>HHHHHHAGFIEDSKASLTLRNFYINTDNRNGTASPSKQEEWGQGFILNYQSGFTQGTVGFGVDALGLLGVRLDGGGRAGKSGLDRQPGTVFPLESNGEPVHDFASLGLTAKAKVSNTEFRYGTLQPKLPVVTYNDGRLLPVTFEGGQVTSTDLKDFTLVAGQLEHSKGRNSTDNRSLSIAGANGSSASSRDSNKFYYAGGDYKVNKDLTLQYYYGNLDDFYKQHFLGLIHNWQIGPGVLKTDLRAFDSSSDGKNGSRSGRADGYVSSGYYGSGVTKGEVDNRAFSGLFTYTV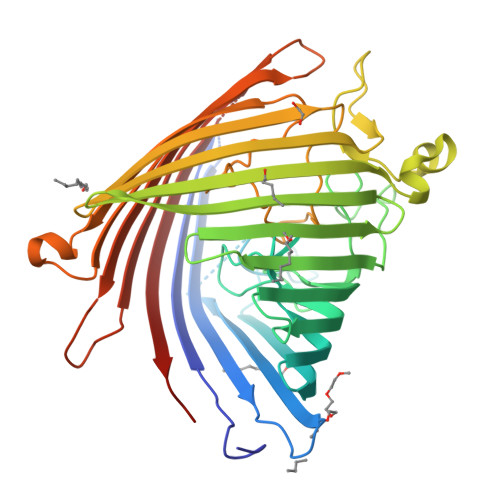SGHSIGAGYQILNGDSDFPFLNRGDGEGSTAYLITDVQIGKFQRAGERTWQVRYGYDFATVGVPGLTFNTIYLSGDKIKTARGDQSEWERDISLAYVIPDGTFKGLGFTWKNASFRSGLPAAGSSNNQRDQDENRLIVSYTLPLL[2x]>[2x]NGIVPDAGHQGPDVSAVNGGTQVINIVTPNNEGISHNQYQDFNVGKPGAVFN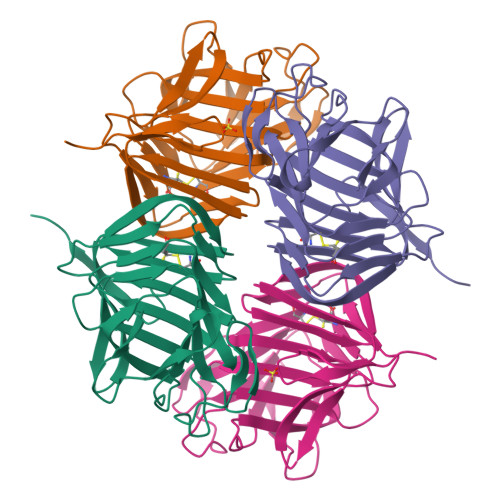NALEAGQSQLAGHLNANSNLNGQAASLILNEVVSRNPSFLLGQQEVFGIAAEAVLSNPNGITCDGCGFINTSRSSLVVGNPLFENGQLKGYSTLNNTNLLSLGKNGLNTTGLLDLIAPRIDSRGKITAAEISAFTGQNTFSQHFDILSSQKPVSALDSYFFGSMQSGRIRIINTAEGSGVKLAGHHHHHH> GGAAAATTT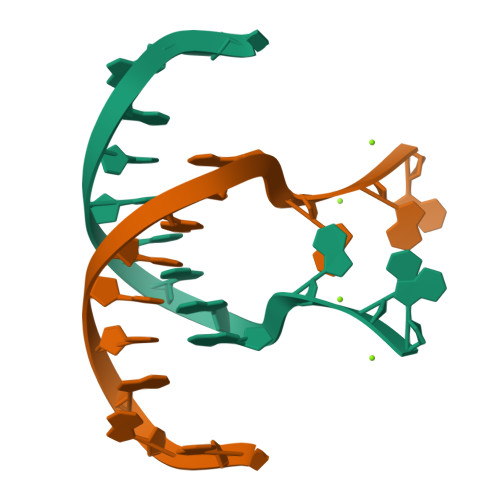GGAG4-[[4-[1,3-bis(oxidanylidene)isoindol-2-yl]phenyl]sulfonylamino]benzoic 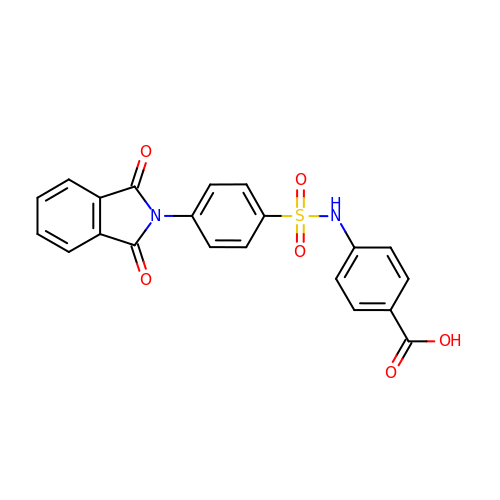acid | C21 H14 N2 O6 S | KCHARURJHJMOQX-UHFFFAOYSA-N>[5x]SNAMIIRPEQHWFLRLFDWHGSVLSKIIFRLLLNVLMSIIAIISYQWYEQLGIHLTVAPFSLLGIAIA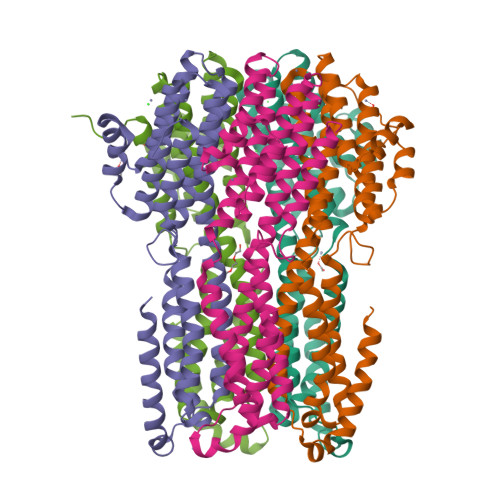IFLGFRNSASYSRFVEARNLWGTVLIAERTLVRQLRNILPAEHDAHRRIVSYLVAFSWSLKHQLRKTDPTADLRRLLPEERVTEILASSMPTNRILLLAGNEIGQLREAAKLSDITYGLMDNKLDELAHVLGGCERLATTPVPFAYTLILQRTVYLFCTLLPFALVGDLHYMTPFVSVFISYTFLSWDSLAEELEDPFGTAANDLPLNAMCNTIERNLLDMTGQHPLPE>[6x]MINEKFPKIWYGGDYNPEQWDKATMEEDMRMFNLAGIDVATVNVFSWAKIQRDEVSYDFTWLDDIIERLTKENIYLCLATSTGAHPAWMAKKYPDVLRVDYEGRKRKFGGRHNSCPNSPTYRKYAKILAGKLAERYKDHPQIVMWHVSNEYGGYCYCDNCEKQFRVWLKERYGTLEALNKAWNTSFWSHTFYDWDEIVAPNALSEEWSGNRTNFQGISLDYRRFQSDSLLECFKMERDELKRWTPDIPVTTNLMGFYPELDYFKWAKEMDVVSWDNYPSMDTPFSFTAMAHNLM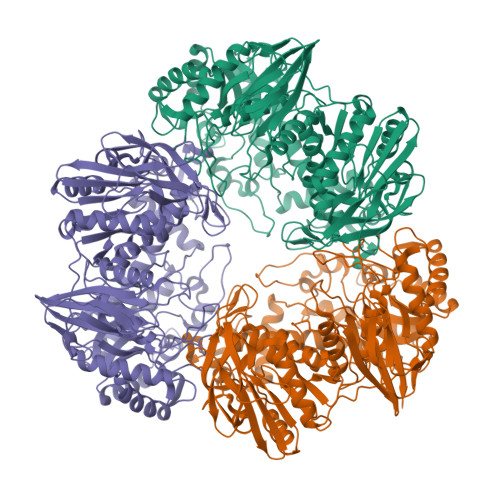RGLKSGQPFMLMEQTPGVQNWQPYNSAKRPGVMRLWSYQAVAHGADTVMFFQLRRSVGACEKYHGAVIEHVGHEHTRVFRECAELGKELQQLGDTILDARSEAKVAVMYDWENRWALELSSGPSIALNYVNEVHKYYDALYKQNIQTDMISVEEDLSKYKVVIAPVMYMVKPGFAERVERFVAQGGTFVTTFFSGIVNENDLVTLGGYPGELRNVMGIWAEEIDALLPGHQNEIVLRQDWGGLRGSYSCGILCDVIHAETAEVLAEYGADYYKGTPVLTRNKFGNGQSYYVASSPDADFLQGLIANLCEEQGVKPLLNTPDGVEVAERVKNGTSYLFVMNHNAEEMTFDAGASRQRDLLTGKTISGQATIPARGVMILERA>MGHHHHHHHHSGDSPAVT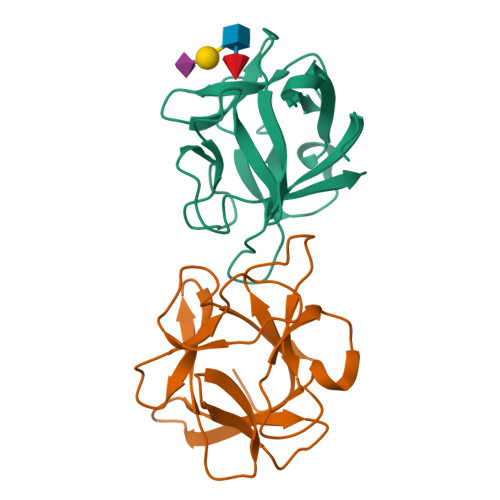LSAGNYIIYNRVLSPRGEKLALTYPGRQRTPVTVSPLDGSSEQAWILRSYDSNSNTWTISPVGSPNSQIGWGAGNVPVVLPPNNYVWTLTLTSGGYNIQDGKRTVSWSLNNATAGEEVSIGADATFSGRWVIEKV[4x]>[2x]YIPEW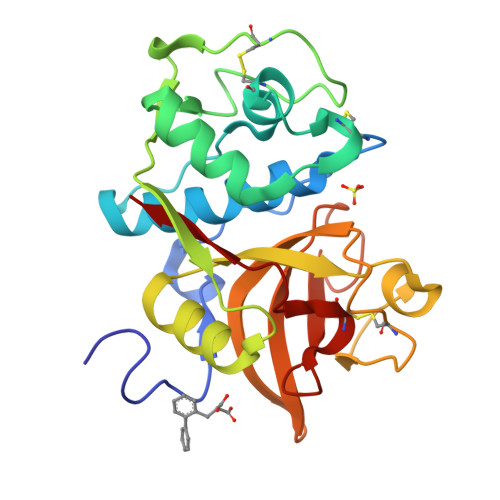EGRAPDSVDYRKKGYVTPVKNQGQCGSSWAFSSVGALEGQLKKKTGKLLNLSPQNLVDCVSENDGCGGGYMTNAFQYVQKNRGIDSEDAYPYVGQEESCMYNPTGKAAKCRGYREIPEGNEKALKRAVARVGPVSVAIDASLTSFQFYSKGVYYDESCNSDNLNHAVLAVGYGIQKGNKHWIIKNSWGENWGNKGYILMARNKNNACGIANLASFPKM(2S,5R,6R,7R)-6-{[(2R)-2-carboxy-2-phenylacetyl]amino}-7-hydroxy-3,3-dimethyl-4-thia-1-azabicyclo[3.2.0]heptane-2-carboxylic 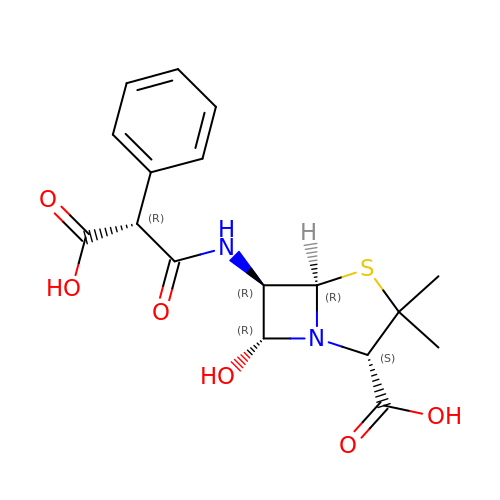acid | C17 H20 N2 O6 S | ASNJKAXIMWOZDG-KHQUWSPVSA-N> MLVDLNVPWPQNSYADKVTSQAVNNLIKTLSTLHMLGYTHIAINFTVNHSEKFPNDVKLLNPIDIKRRFGELMDRTGLKLYSRITLIIDDPSKGQSLSKISQAFDIVAALPISEKGLTLSTTNLDIDLLTFQYGSRLPTFLKHKSICSCVNRGVKLEIVYG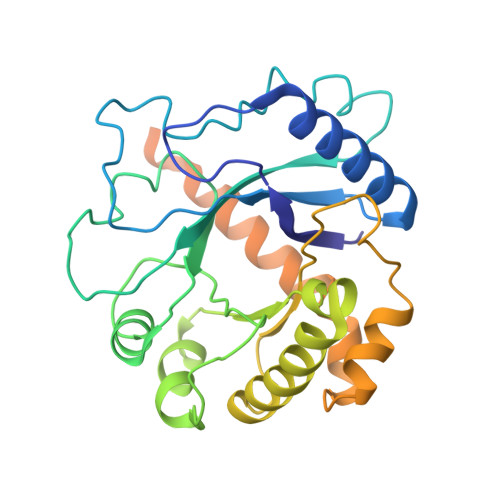YALRDVQARRQFVSNVRSVIRSSRSRGIVIGSGAMSPLECRNILGVTSLIKNLGLPSDRCSKAMGDLASLVLLNGRLRNKSHKQTIVTGGGSGNGDDVVNDVQGIDDVQTIKVVKRSMDAEQLGHASKRHKP2-pyren-1-yloxyethyl 2-[1,5-dimethyl-2,4-bis(oxidanylidene)-6-(2-oxidanyl-6-oxidanylidene-cyclohexen-1-yl)carbonyl-quinazolin-3-yl]ethanoate 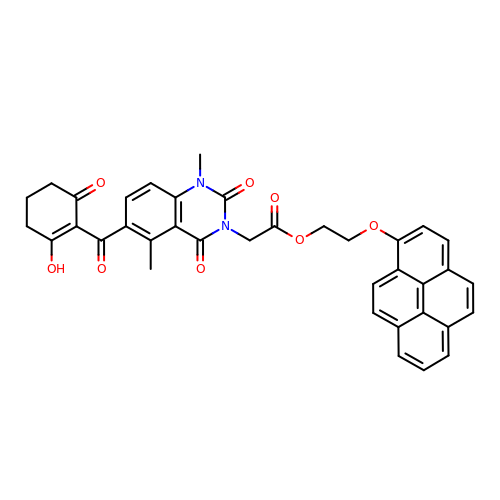| C37 H30 N2 O8 | VGRDNFRONVWWKB-UHFFFAOYSA-N> MLGSGFKAERLRVNLRLVINRLKLLEKKKTELAQKARKEIADYLAAGKDERARIRVEHI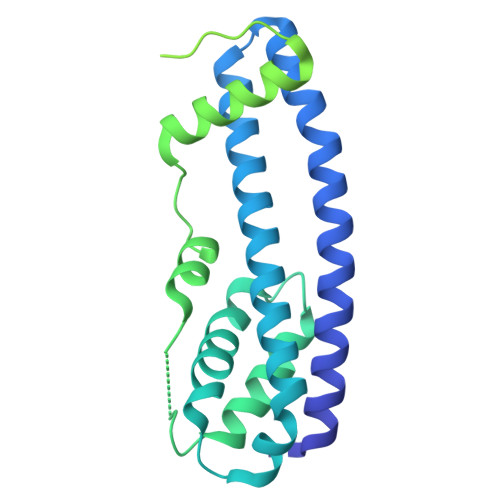IREDYLVEAMEILELYCDLLLARFGLIQSMKELDSGLAESVSTLIWAAPRLQSEVAELKIVADQLCAKYSKEYGKLCRTNQIGTVNDRLMHKLSVEAPPKILVERYLIEIAKNYNVPYEPDSVVMAEAPPGVETDLIDVGFTDDVKKGGPGRGGSGGFTAPVGGPDGTVPMPMPMPMPMPSANTPFSYPLPKGPSDFNGLPMGTYQAFPNIHPPQIPATPPSYESVDDINADKNISSAQIVGPGPKPEASAKLPSRPADNYDNFVLPELPSVPDTLPTASAGASTSASEDIDFDDLSRRFEELKKKT>MDVSKRPREEFHKEQCLSFVKKLWAADTLAMFHYPVSATEVPGYYDVVDTPMDLSTIRKNIEQGKYRTDTEVENDVVLMLSNALDFNEKGSQWHDLAKQ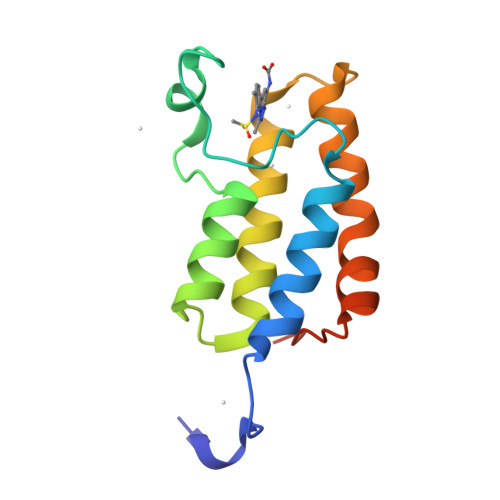LKKRYLTLAQESGLSFDADQAFIPTK[2x]>MDYKDDDDKLAAANSSIDLISTSLYKKAGLTMVTGGGAAPPGTVTEPLPSVIVLSAGRKMAAAAAAASGPGCSSAAGAGAAGVSEWLVLRDGCMHCDADGLHSLSYHPALNAILAVTSRGTIKVIDGTSGATLQASALSAKPGGQVKCQYISAVDKVIFVDDYAVGCRKDLNGILLLDTALQTPVSKQDDVVQLELPVTEAQQLLSACLEKVDISSTEGYDLFITQLKDGLKNTSHETAANHKVAKWATVTFHLPHHVLKSIASAIVNELKKINQNVAALPVASSVMDRLSYLLPSARPELGVGPGRSVDRSLMYSEANRRETFTSWPHVGYRWAQPDPMAQAGFYHQPASSGDDRAMCFTCSVCLVCWEPTDEPWSEHERHSPNCPFVKGEHTQNVPLSVTLATSPAQFPCTDGTDRISCFGSGSCPHFLAAATKRGKICIWDVSKLMKVHLKFEINAYDPAIVQQLILSGDPSSGVDSRRPTLAWLEDSSSCSDIPKLEGDSDDLLEDSDSEEHSRSDSVTGHTSQKEAMEVSLDITALSILQQPEKLQWEIVANVLEDTVKDLEELGANPCLTNSKSEKTKEKHQEQHNIPFPCLLAGGLLTYKSPATSPISSNSHRSLDGLSRTQGESISEQGSTDNESCTNSELNSPLVRRTLPVLLLYSIKESDEKAGKIFSQMNNIMSKSLHDDGFTVPQIIEMELDSQEQLLLQDPPVTYIQQFADAAANLTSPDSEKWNSVFPKPGTLVQCLRLPKFAEEENLCIDSITPCADGIHLLVGLRTCPVESLSAINQVEALNNLNKLNSALCNRRKGELESNLAVVNGANISVIQHESPADVQTPLIIQPEQRNVSGGYLVLYKMNYATRIVTLEEEPIKIQHIKDPQDTITSLILLPPDILDNREDDCEEPIEDMQLTSKNGFEREKTSDISTLGHLVITTQGGYVKILDLSNFEILAKVEPPKKEGTEEQDTFVSVIYCSGTDRLCACTKGGELHFLQIGGTCDDIDEADILVDGSLSKGIEPSSEGSKPLSNPSSPGISGVDLLVDQPFTLEILTSLVELTRFETLTPRFSATVPPCWVEVQQEQQQRRHPQHLHQQHHGDAAQHTRTWKLQTDSNSWDEHVFELVLPKACMVGHVDFKFVLNSNITNIPQIQVTLLKNKAPGLGKVNALNIEVEQNGKPSLVDLNEEMQHMDVEESQCLRLCPFLEDHKEDILCGPVWLASGLDLSGHAGMLTLTSPKLVKGMAGGKYRSFLIHVKAVNERGTEEICNGGMRPVVRLPSLKHQSNKGYSLASLLAKVAAGKEKSSNVKNENTSGTRKSENLRGCDLLQEVSVTIRRFKKTSISKERVQRCAMLQFSEFHEKLVNTLCRKTDDGQITEHAQSLVLDTLCWLAGVHSNGPGSSKEGNENLLSKTRKFLSDIVRVCFFEAGRSIAHKCARFLALCISNGKCDPCQPAFGPVLLKALLDNMSFLPAATTGGSVYWYFVLLNYVKDEDLAGCSTACASLLTAVSRQLQDRLTPMEALLQTRYGLYSSPFDPVLFDLEMSGSSCKNVYNSSIGVQSDEIDLSDVLSGNGKVSSCTAAEGSFTSLTGLLEVEPLHFTCVSTSDGTRIERDDAMSSFGVTPAVGGLSSGTVGEASTALSSAAQVALQSLSHAMASAEQQLQVLQEKQQQLLKLQQQKAKLEAKLHQTTAAAAAAASAVGPVHNSVPSNPVAAPGFFIHPSDVIPPTPKTTPLFMTPPLTPPNEAVSVVINAELAQLFPGSVIDPPAVNLAAHNKNSNKSRMNPLGSGLALAISHASHFLQPPPHQSIIIERMHSGARRFVTLDFGRPILLTDVLIPTCGDLASLSIDIWTLGEEVDGRRLVVATDISTHSLILHDLIPPPVCRFMKITVIGRYGSTNARAKIPLGFYYGHTYILPWESELKLMHDPLKGEGESANQPEIDQHLAMMVALQEDIQCRYNLACHRLETLLQSIDLPPLNSANNAQYFLRKPDKAVEEDSRVFSAYQDCIQLQLQLNLAHNAVQRLKVALGASRKMLSETSNPEDLIQTSSTEQLRTIIRYLLDTLLSLLHASNGHSVPAVLQSTFHAQACEELFKHLCISGTPKIRLHTGLLLVQLCGGERWWGQFLSNVLQELYNSEQLLIFPQDRVFMLLSCIGQRSLSNSGVLESLLNLLDNLLSPLQPQLPMHRRTEGVLDIPMISWVVMLVSRLLDYVATVEDEAAAAKKPLNGNQWSFINNNLHTQSLNRSSKGSSSLDRLYSRKIRKQLVHHKQQLNLLKAKQKALVEQMEKEKIQSNKGSSYKLLVEQAKLKQATSKHFKDLIRLRRTAEWSRSNLDTEVTTAKESPEIEPLPFTLAHERCISVVQKLVLFLLSMDFTCHADLLLFVCKVLARIANATRPTIHLCEIVNEPQLERLLLLLVGTDFNRGDISWGGAWAQYSLTCMLQDILAGELLAPVAAEAMEEGTVGDDVGATAGDSDDSLQQSSVQLLETIDEPLTHDITGAPPLSSLEKDKEIDLELLQDLMEVDIDPLDIDLEKDPLAAKVFKPISSTWYDYWGADYGTYNYNPYIGGLGIPVAKPPANTEKNGSQTVSVSVSQALDARLEVGLEQQAELMLKMMSTLEADSILQALTNTSPTLSQSPTGTDDSLLGGLQAANQTSQLIIQLSSVPMLNVCFNKLFSMLQVHHVQLESLLQLWLTLSLNSSSTGNKENGADIFLYNANRIPVISLNQASITSFLTVLAWYPNTLLRTWCLVLHSLTLMTNMQLNSGSSSAIGTQESTAHLLVSDPNLIHVLVKFLSGTSPHGTNQHSPQVGPTATQAMQEFLTRLQVHLSSTCPQIFSEFLLKLIHILSTERGAFQTGQGPLDAQVKLLEFTLEQNFEVVSVSTISAVIESVTFLVHHYITCSDKVMSRSGSDSSVGARACFGGLFANLIRPGDAKAVCGEMTRDQLMFDLLKLVNILVQLPLSGNREYSARVSVTTNTTDSVSDEEKVSGGKDGNGSSTSVQGSPAYVADLVLANQQIMSQILSALGLCNSSAMAMIIGASGLHLTKHENFHGGLDAISVGDGLFTILTTLSKKASTVHMMLQPILTYMACGYMGRQGSLATCQLSEPLLWFILRVLDTSDALKAFHDMGGVQLICNNMVTSTRAIVNTARSMVSTIMKFLDSGPNKAVDSTLKTRILASEPDNAEGIHNFAPLGTITSSSPTAQPAEVLLQATPPHRRARSAAWSYIFLPEEAWCDLTIHLPAAVLLKEIHIQPHLASLATCPSSVSVEVSADGVNMLPLSTPVVTSGLTYIKIQLVKAEVASAVCLRLHRPRDASTLGLSQIKLLGLTAFGTTSSATVNNPFLPSEDQVSKTSIGWLRLLHHCLTHISDLEGMMASAAAPTANLLQTCAALLMSPYCGMHSPNIEVVLVKIGLQSTRIGLKLIDILLRNCAASGSDPTDLNSPLLFGRLNGLSSDSTIDILYQLGTTQDPGTKDRIQALLKWVSDSARVAAMKRSGRMNYMCPNSSTVEYGLLMPSPSHLHCVAAILWHSYELLVEYDLPALLDQELFELLFNWSMSLPCNMVLKKAVDSLLCSMCHVHPNYFSLLMGWMGITPPPVQCHHRLSMTDDSKKQDLSSSLTDDSKNAQAPLALTESHLATLASSSQSPEAIKQLLDSGLPSLLVRSLASFCFSHISSSESIAQSIDISQDKLRRHHVPQQCNKMPITADLVAPILRFLTEVGNSHIMKDWLGGSEVNPLWTALLFLLCHSGSTSGSHNLGAQQTSARSASLSSAATTGLTTQQRTAIENATVAFFLQCISCHPNNQKLMAQVLCELFQTSPQRGNLPTSGNISGFIRRLFLQLMLEDEKVTMFLQSPCPLYKGRINATSHVIQHPMYGAGHKFRTLHLPVSTTLSDVLDRVSDTPSITAKLISEQKDDKEKKNHEEKEKVKAENGFQDNYSVVVASGLKSQSKRAVSATPPRPPSRRGRTIPDKIGSTSGAEAANKIITVPVFHLFHKLLAGQPLPAEMTLAQLLTLLYDRKLPQGYRSIDLTVKLGSRVITDPSLSKTDSYKRLHPEKDHGDLLASCPEDEALTPGDECMDGILDESLLETCPIQSPLQVFAGMGGLALIAERLPMLYPEVIQQVSAPVVTSTTQEKPKDSDQFEWVTIEQSGELVYEAPETVAAEPPPIKSAVQTMSPIPAHSLAAFGLFLRLP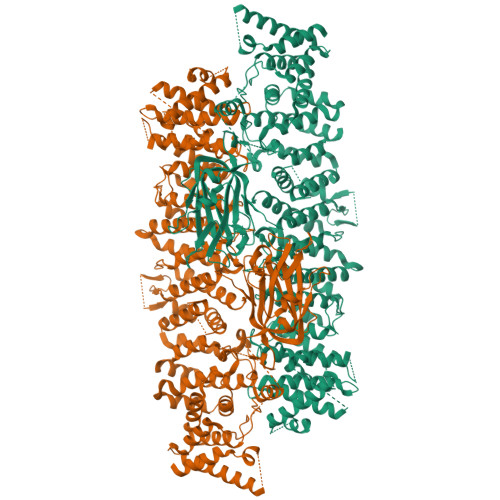GYAEVLLKERKHAQCLLRLVLGVTDDGEGSHILQSPSANVLPTLPFHVLRSLFSTTPLTTDDGVLLRRMALEIGALHLILVCLSALSHHSPRVPNSSVNQTEPQVSSSHNPTSTEEQQLYWAKGTGFGTGSTASGWDVEQALTKQRLEEEHVTCLLQVLASYINPVSSAVNGEAQSSHETRGQNSNALPSVLLELLSQSCLIPAMSSYLRNDSVLDMARHVPLYRALLELLRAIASCAAMVPLLLPLSTENGEEEEEQSECQTSVGTLLAKMKTCVDTYTNRLRSKRENVKTGVKPDASDQEPEGLTLLVPDIQKTAEIVYAATTSLRQANQEKKLGEYSKKAAMKPKPLSVLKSLEEKYVAVMKKLQFDTFEMVSEDEDGKLGFKVNYHYMSQVKNANDANSAARARRLAQEAVTLSTSLPLSSSSSVFVRCDEERLDIMKVLITGPADTPYANGCFEFDVYFPQDYPSSPPLVNLETTGGHSVRFNPNLYNDGKVCLSILNTWHGRPEEKWNPQTSSFLQVLVSVQSLILVAEPYFNEPGYERSRGTPSGTQSSREYDGNIRQATVKWAMLEQIRNPSPCFKEVIHKHFYLKRVEIMAQCEEWIADIQQYSSDKRVGRTMSHHAAALKRHTAQLREELLKLPCPEGLDPDTDDAPEVCRATTGAEETLMHDQVKPSSSKELPSDFQL[2x]1, 4-Dihydroxy-2-naphthoyl-CoA (DHNA-CoA) synthase, also called MenB, is responsible for conversion of o-succinylbenzoyl-CoA to DHNA-CoA in the biosynthesis of both vitamin K1 and K2. It catalyzes a multiple-step intramolecular Claisen condensation reaction involving two high energy oxyanion intermediates and two keto-enol tautomerizations in the formation of a naphthenoid ring. The first crystal structure of DHNA-CoA synthase from Mycobacterium tuberculosis shows that it forms two eclipsed trimers organized in a homologous hexameric assembly, in which each monomer is comprised of an N-terminal spiral core domain and a C-terminal helical domain conforming to a canonical crotonase fold. In addition to observing the folding of the active-site loop into a well-defined structure as previously seen in the substrate analog complex structure, we have identified a significant reorientation of the C-terminal helix as an additional conformational change caused by the small molecule ligands.

There are two hexamers in an asymmetric unit of the ecMenB: HNA-CoA complex structure with their three-fold axes tilted with each other at an angle of <5°, similar to the arrangement of two hexamers in the asymmetric unit of the crystal of Mycobacterium tuberculosis MenB in complex with acetoacetyl-CoA. All subunits in one hexamer are saturated with the ligand in 1∶1 ratio and overlap very well with each other with a rmsd <0.18 Å over all Cα atoms, whereas only five subunits in the other hexamer bind HNA-CoA and no electron density of the ligand is found in the sixth subunit (chain D). The other structural change is a significant reorientation of the C-terminal helix (called C-helix, residues 260–272) of the opposing subunit by an angle of ∼15° towards the enzyme active site. These structural effects of the ligand binding are best demonstrated by comparing the structure of the unliganded subunit (chain D) with its opposing, liganded subunit (chain B) across the trimer-trimer interface in the second hexamer. The unliganded subunit has a disordered A-loop and its C-helix is bent towards the active site of the opposing subunit with the small molecule ligand. In contrast, the liganded subunit contains the ordered A-loop and its C-helix is not bent towards the empty active site of the unliganded subunit. These structural differences between the two opposing subunits provide unambiguous evidence that the observed conformational changes are induced by binding of the small molecule ligand. The conserved active-site residues in ecMenB: HNA-CoA take the same positions and orientations as those in the previously reported ecMenB: OSB-NCoA structure, despite the obvious structural difference in the small molecule ligands.

>MIYPDEAMLYAPVEWHDCSEGFEDIRYEKSTDGIAKITINRPQVRNAFRPLTVKEMIQALADARYDDNIGVIILTGAGDKAFCSGGDQKVRGDYGGYKDDSGVHHLNVLDFQRQIRTCPKPVVAMVAGYSIGGGHVLHMMCDLTIAADNAIFGQTGPKVGSFDGGWGASYMARIVGQKKAREIWFLCRQYDAKQALDMGLVNTVVPLADLEKETVRWCREMLQNSPMALRCLKAALNADCDGQAGLQELAGNATMLFYMTEEGQEGRNAFNQKRQPDFSKFKRNP[12x]> GHR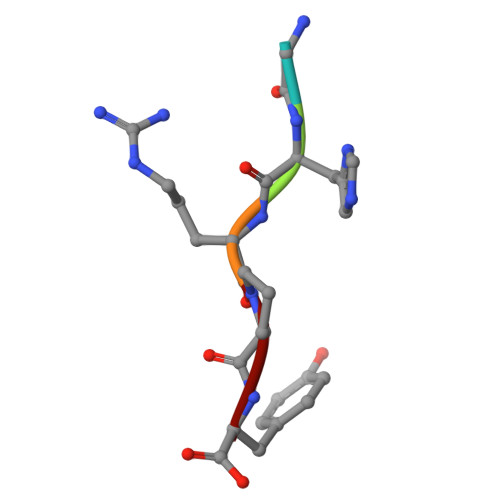PY(4~{S})-5-[4-[[4-(2-ethyl-2-oxidanyl-butoxy)-2-methyl-phenyl]-dimethyl-silyl]-3-methyl-phenoxy]-4-oxidanyl-pentanoic 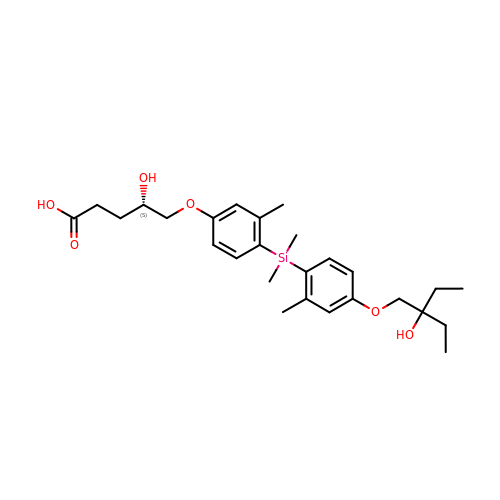acid | C27 H40 O6 Si | OSYCNJSNXPMJRY-NRFANRHFSA-N> PSIKSGTILHAWNWSFNTLKNNMKDIHDAGYTAIQTSPINQVKEGNKGDKSMGNWYWLYQPTSYQIGNRYLGSEEEFKEMCAAAEEYGVKVIVDAVINHTTSDYAAISNEIKSISNWTHGNTQIKNWSDRWDVTQNSLLGLYDWNTQNTQVQSYLKRFLERALNDGADGFRYDAAKHIELPDDGNYGSQFWPNITNTSAEFQYGEILQDSASRDAAYANYMNVTASNYGHSIRSALKNRNLSVSNISHYASDVSADKLVTWVESHDTYANDDEESTWMS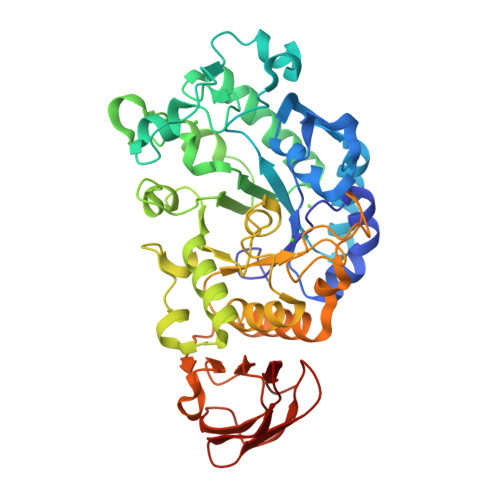DDDIRLGWAVIASRSGSTPLFFSRPDGGGNGVRFPGKTQIGDRGSALFEDQAIVAVNTFHNVMAGQPEELSNPNGNNQIFMNQRGSKGVVLANAGSSSVSINASTKLPDGSYDNKAGTGSFQVRDGKLTGTINARSVAVLYPD> GHMAFSNPFDDPQGAFYILRNAQGQFSLWPQQC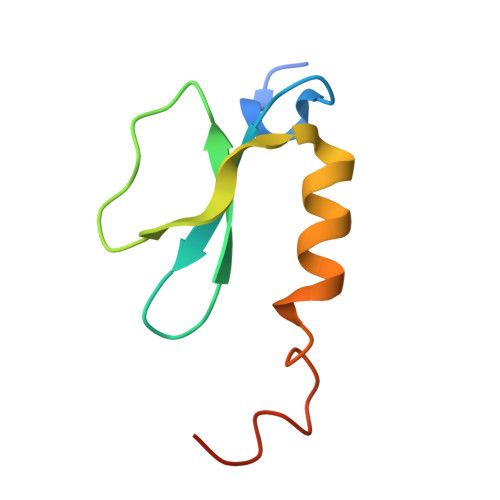VLPAGWDIVCQPQSQASCQQWLEAHWRTLTPTNFTQLQEAQ> MTNATIAPTTTAAPVTKSVDAPTADENTPLFSPSLISPDVLAVLPADYTIRPLCRSDYKRGYLDVLRVLTTVGDINEEQWNSRYEWIRARSDEYYLLVVCDGEGRIVGTGSLVVERKFIHSLGMVGHIEDIAVEKGQQGKKLGLRIIQALDYVAEKVGCYKTILDCSEANEGFYIKCGFKRAGLEMAHYY

Gna1 (EC 2.3.1.4) is a member of the Gcn5-related N-acetyltransferase (GNAT) superfamily and is present in yeast such as Candida spp. (e.g. Candida albicans, Candida glabrata, and Candida auris) and Saccharomyces cerevisiae. Mechanistically, A. fumigatus (Af) Gna1 facilitates N-acetylation of GlcN-6P by promoting direct nucleophilic attack at the thioester carbonyl group of the acetyl coenzyme A (AcCoA) cofactor by the sugar-phosphate amino group. Previous work has shown that A. fumigatus Gna1 possesses a classic GNAT α/β-fold, forming an obligate homodimer. This dimer shows extensive secondary structure swapping with substrate and cofactor binding to the two active sites that are formed by channels on the surface of the enzyme, composed of amino acids from both AfGna1 monomers.

As an alternative approach to achieving AfGna1 inhibition, we aimed to exploit the protein tunnels that connect the dimer interface fragment binding pocket to the substrate-binding sites (distance of 1 to substrate-binding site = ∼8 Å). Extension of the fragment scaffold into the active sites by traversing these tunnels would effectively generate a competitive enzyme inhibitor by blocking substrate binding at both AfGna1 active sites (bifurcation approach). To test the ability of a bifurcated derivative of 1 to bind AfGna1, 3 was synthesized. This bifurcated fragment introduces an N,N-diethyl alcohol moiety into the scaffold and displays a binding affinity of the same order as fragment hit 1 (5 μm). An AfGna1–3 complex structure, which additionally contains Glc-6P, indicates that 3 is accessible to the fragment-binding site, despite narrow tunnels linking the fragment binding pocket to the enzyme active sites. Like fragment hit 1 and 2, the important binding interactions and binding mode are maintained in the AfGna1–3-(Glc-6P) complex structure. In addition, the hydroxy functionality of the N,N-diethyl alcohol moiety displaces His-127–coordinating water molecules and interacts with the acceptor nitrogen atoms of the His-127 side chains. The introduction of a para-anilino anchoring point for bifurcation leverages the sp2 character of the anilino-nitrogen, maintaining the planarity necessary at the branch point for correct N,N-diethyl alcohol orientation whereas ortho-dichloro substitution positions the fragment along the 2-fold crystallographic axis (with a positional shift of 0.6 Å and 19° reorientation from fragment hit 1). Moreover, the positioning of the Glc-6P 6.2 Å from the ethyl chain linker of 3, visible in the AfGna1–3-(Glc-6P) complex structure, is suggestive of fragment-linking approaches toward AfGna1 inhibition, albeit challenging because of the limited size of the tunnel. In line with this, derivative 3 did not show inhibition against AfGna1 in a recombinant enzyme assay, probably because of the inability of the N,N-diethyl alcohol moiety to extend into and block the enzyme active sites.>MTPAPTPRTDQLHGSRVLVIG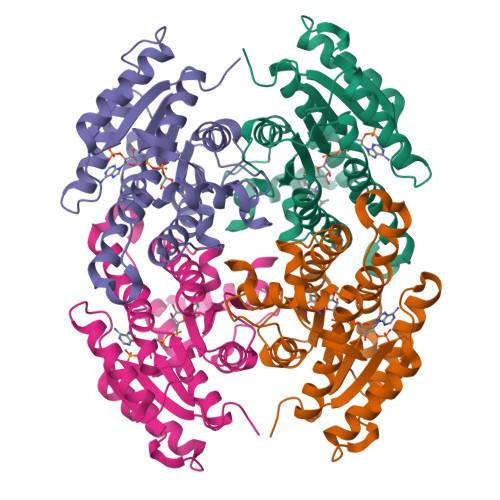GTSGIGFAVCAAALGHGAIVTIVGSNAQKLKDSVARLKSSFPSTDPDDIVAVRCDLSNSDTVEQDIEKALQLAAGNSKINHIVITAADMTAPPPLEDLTVDSVQRPGIIRLVAPLMVAKHLPKYMNKCPQSSLTLTSGAHCLRPNPGWTVISGYCGAVEAMSRGLAIDLKPLRVNVVAPGAVLTEAVKDILGDAYDAAVEMAEAKSTVGQTGSPESVAQAYIYLMKDHYASGSVVSTNGGMLLV[6x]> GPMEVDSILGSLSITDDFDQLVDVTSLFDELCSKLKPEAIVKDPRFDLFEGTHSLEVNNSKLDSSLIELTAEEIEFDVNVAYDPPLASVAAIADRLLRCVISWLNDYQTLPTTVLSCRYTESLLSSLVKGTTAGSSWCTGNILYDKVLGSCILGVCYLTKFVQKLLSAGIVFEEEDLNFNNMGFNTFDNLPGQDVVINSLTESLQILEAYSDDSLHLTMLKHILKIIICLVHLEDHLTDYSTKTSHLDELIENANSVNGIFPQLQLSPPKGAFSTYIQKHRSNQFPPRKITKLP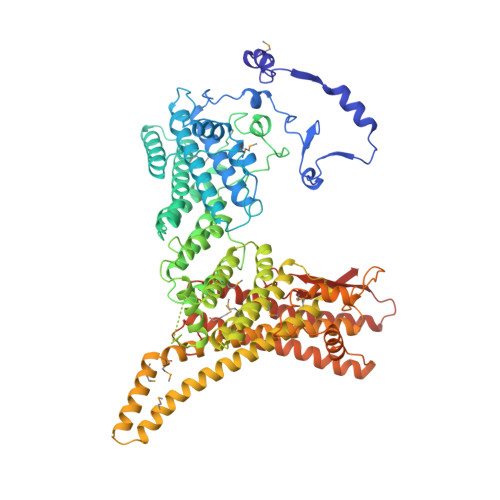TDYSGFITLANDVKTILLVDKAESALETYQFAKFFNKLEQRHVIARILFPLFFIRDDRTVLGKFSYTQFYLLHVKEFSAQTPSEFESSIGNELIQESSNMLLEWYQNCSQNTCRYRQGFNRQLILWDSLQAQFESVNSQVYCSWTYFMKLSSMIEFSLKGFDLDIYKPFEAYSMFWYVYYLSHHLETFLKDSQNDIESNINAIHSMNKKLKKLKAGEKKDQLRLKYRFAMDNEMEQLQATKQFLNYLLKEINITKSLCLIEVFQFAILKSFGLIDNKNSTPSKFSNERLIHNLRFKPFNSIGVPELPEYEVFQQTLKDFVIEEKGAAFDIKLERATNFIETEVRNVVSSIDEIMQGIKGGDNNGVLVTGTRLVQELSLEYYCKLKHTSKALSVNSKVIVNTLKKNIKNKDSHEYKVELVHTTEGWNYFPIQTLRIKQDRYK> MTENILRKSDEEIQKEITARVKALESMLIEQGILTTSMIDRMAEIYENEVGPHLGAKVVVKAWTDPEFKKRLLADGTEACMTENILRKSDEEIQKEITARVKALESMLIEQGILTTSMIDRMAEIYENEVGPHLGAKVVVKAWTDPEFKKRLLADGTEACKELGIGGLQGEDMMWVENTDEVHHVVVCTLCSCYPWPVLGLPPNWFKEPQYRSRVVREPRQLLKEEFGFEVPPSKEIKVWDSSSEMRFVVLPQRPAGTDGWSEEELATLVTRESMI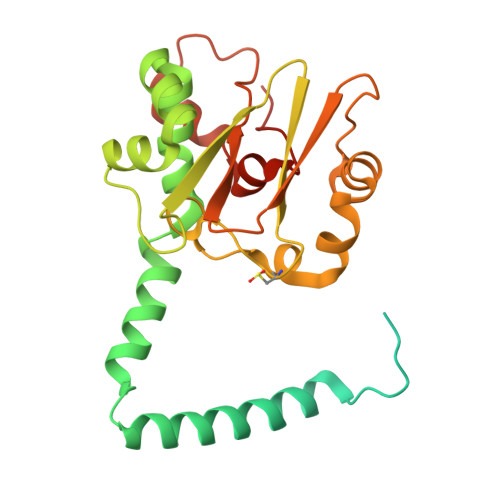GVEPAKAVHHHHHH>MGSSHHHHHHSSGRENLYFQGHMLFISATNTNAGKTTCARLLAQYCNACGVKTILLKPIETGVNDAINHSSDAHLFLQDNRLLDRSLTLKDISF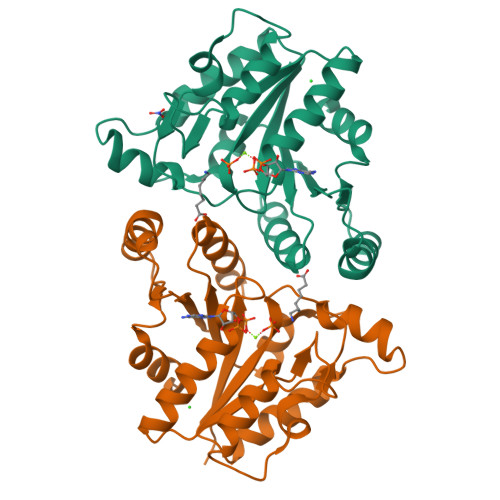YRYHKVSAPLIAQQEEDPNAPIDTDNLTQRLHNFTKTYDLVIVEGAGGLCVPITLEENMLDFALKLKAKMLLISHDNLGLINDCLLNDFLLKSHQLDYKIAINLKGNNTAFHSISLPYIELFNTRSNNPIVIFQQSLKVLMSFALKGS[6x]> KDTIALVVSTLNNPFFVSLKDGAQKEADKLGYNLVVLDSQNNPAKELANVQDLTVRGTKILLINPTDSDAVGNAVKMANQANIPVITLDRQATKGEVVSHIASDNVLGGKIAGDYIAKKAGE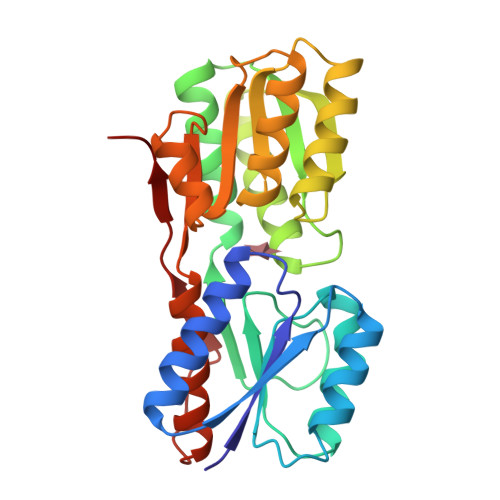GAKVIELQGIARTSAARERGEGFQQAVAAHKFNVLASQPADFDRIKGLNVMQNLLTAHPDVQAVFAQNDEMALGALRALQTAGKSDVMVVGFDGTPDGEKAVNDGKLAATIAQLPDQIGAKGVETADKVLKGEKVQAKYPVDLKLVVKQ>[2x]GSVDSVLFGSLRGHVVGLRYYTGVVNNNEMVALQRDPNNPYDKNAIKVNNVNGNQVGHLKKELAGALAYIMDNKLAQIEGVVPFGANNAFTMPLHMT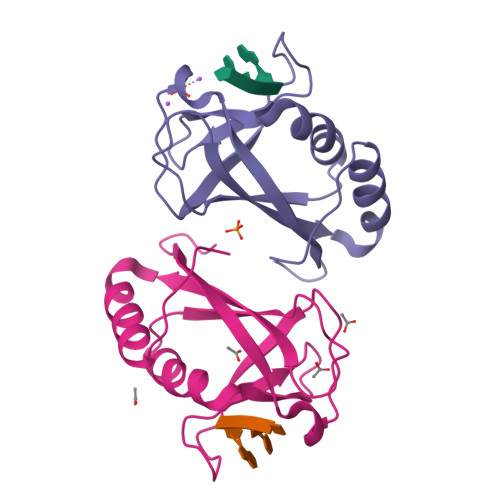FWGKEENRKAVSDQLKKHGFKLGPAP> SGSREPNLFRSLVGTSRAIQQVRQMMQQV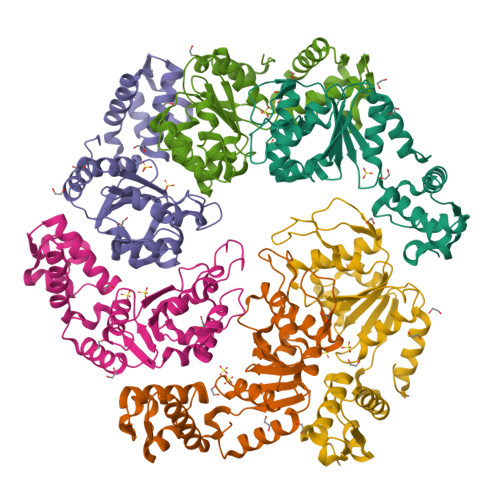ADTDASVLILGESGTGKEVVARNLHYHSKRREGPFVPVNCGAIPAELLESELFGHEKGAFTGAITSRAGRFELANGGTLFLDEIGDMPLPMQVKLLRVLQERTFERVGSNKTQNVDVRIIAATHKNLEKMIEDGTFREDLYYRLNVFPIEMAPLRERVEDIALLLNELISRMEHEKRGSIRFNSAAIMSLCRHDWPGNVRELANLVERLAIMHPYGVIGVGELPKKFRHVD>GAASDVPIRRREEAYENQRWNPMGGFCEKLLLSDRWGWSDVSGLQHRPLDRVALPSPHWEWESD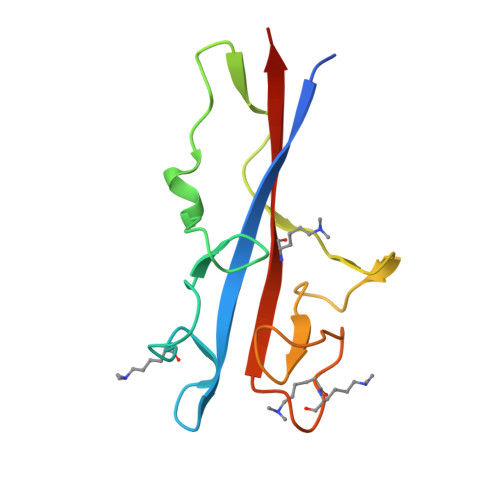WYVDENFGGEPTEKGGWTYAIDFPATYTKDKKWNSCVRRRKWIRYRRYKSRD[3x]>NDLSGKTVIITGGARGLGAEAARQAVAAGARVVLADVLDEEGAATARELGDAARYQHLDVTIEEDWQRVVAYAREEFGSVDGLVNNAGISTGMFLETESVERFRKVVEINLTGVFIGMKTVIPAMKDAGGGSIVNISSAAGLMGL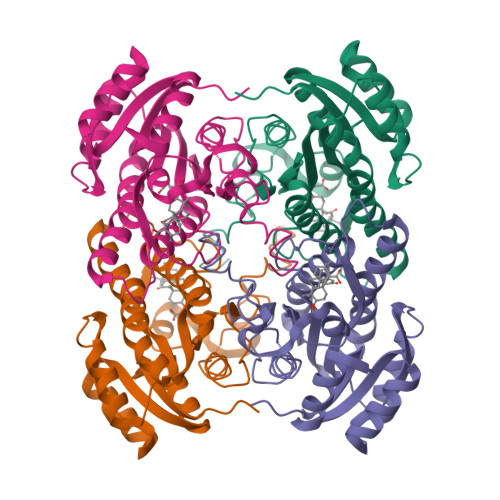ALTSSYGASKWGVRGLSKLAAVELGTDRIRVNSVHPGMTYTPMTAETGIRQGEGNYPNTPMGRVGNEPGEIAGAVVKLLSDTSSYVTGAELAVDGGWTTGPTVKYVMGQ[4x]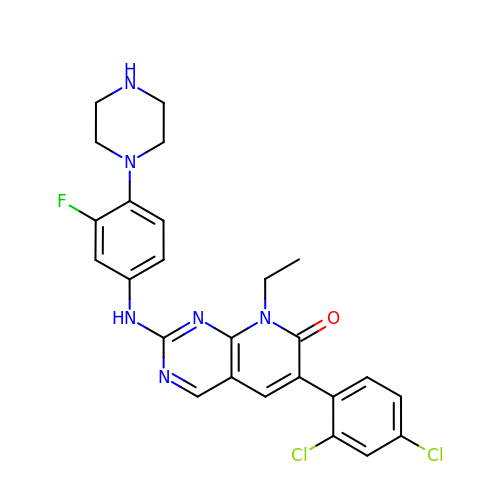6-(2,4-dichlorophenyl)-8-ethyl-2-{[3-fluoro-4-(piperazin-1-yl)phenyl]amino}pyrido[2,3-d]pyrimidin-7(8H)-one | C25 H23 Cl2 F N6 O | DHKFOIHIUYFSOF-UHFFFAOYSA-N> MDDLKLPRQRVDLVAPPFVHVHEQATKQGPKIMEFKLVVQEKKMVIDEKGTTFQAMTFNGSMPGPLMVVHEGDYVEVTLVNPATNTMPHNIDFHSATGALGGGALTLINPGEQVVLRWKATRTGVFVYHCAPGGPMIPWHVVSGMNGAVMVLPRDGLNDGHGHSLRYDRIYYIGEQDLYVPRDEKGNFKSYDSPGEAYSDTEEVMRKLTPTHVVFNGKAGALTGKNALNANVGENVLIVHSQANRDSRPHLIGGHGDYVWETGKFSNAPETGLETWFIRGGSAGAALYKFLQPGIYAYVTHNLIEAANLGATAHFKVEGKWNDDLMTQVKAPADIPTGSTNENLYFQ

We have recently identified a blue CuNiR from Bradyrhizobium ORS 375 of the order Rhizobiales (Br2DNiR). CuNiRs, encoded by the nirK gene, are key enzymes in the denitrification pathway, as it is at this point that the bioavailable fixed nitrogen gets recycled back to the atmosphere. These redox-active metalloenzymes are responsible for catalyzing the one-electron and two-proton reduction of NO2− to gaseous product NO in the first committed step of this pathway (NO2− + 2H+ + e−→NO + H2O). CuNiRs are a highly conserved enzyme family that use cupredoxin-like domains to assemble a catalytic core made up of type 1 Cu (T1Cu) and type 2 Cu (T2Cu). Two invariant active-site pocket residues AspCAT and HisCAT are involved in substrate binding and provision of protons during catalysis, and a conserved IleCAT residue provides steric control of ligand binding to the T2Cu.

To characterize this new two-domain CuNiR enzyme, we obtained a 1.1 Å atomic-resolution structure in its as-isolated state using conventional synchrotron-radiation crystallography (SRX) at 100 K. To provide rigor and reduce the ambiguities in the assignments of multiple conformations of active-site ligands and define SDs of individual bond distances and angles of residues in the catalytic core, we used SHELX-97 [estimated standard deviation (e.s.d.) values available from SHELX are given in brackets]. A notable observation was the presence of two waters: (W1) and (W2) concurrently bound to the catalytic T2Cu site in one conformation and an alternative water (W3) in second conformation. Two waters, W1 and W2, with equal occupancies (0.67) are 2.49 Å apart and bound to the T2Cu atom at distances of 1.940(3) Å and 2.162(3) Å, respectively. The occupancies of ~0.7 for these two waters strongly argue for their coexistence rather than alternate conformations of the same water. An alternative third water, W3, bound at 2.018(3) Å with ideal tetrahedral geometry to T2Cu with an occupancy of 0.33 represents the site in molecules where both W1 and W2 are absent. The catalytically important AspCAT residue (Asp92) is present in both the main (occupancy, 0.67) and distorted (occupancy, 0.33) conformations of its proximal position, as first seen in XFEL structures of AcNiR, with these facing toward the T2Cu site. Although seen together in our atomic-resolution structure, these two AspCAT conformations do not occur simultaneously but are only present either alongside W1 and W2 (main conformation) or alongside W3 (distorted conformation). In its main conformation, the carboxyl oxygen (Oδ2) atom of AspCAT is hydrogen bonded with water W1 and a substrate channel water (W4) with 0.5 occupancy at distances 2.52 and 2.45 Å, respectively, while Oδ2 atom of the distorted conformation is bound to W3 (3.13 Å). The catalytically important HisCAT residue (His250) has its imidazole ring rotated toward Glu274 forming a strong hydrogen bond by its Nδ1 atom with the main-chain carbonyl oxygen of Glu274 at 2.67 Å.> GPMKASLTFSLSGIYAPCSISRDIYLEYGDKKAECLYGTIRLPQYGPGCTPGKIVHCVLDDSLPFCSIVVPSKLFGFMPTQPTMDFCYFEPILDNVVPVLDSVTFLINEQLYSKLMDLPQEMQQIQFLHYKYNINSMETVVHSRDILTSGLCQILN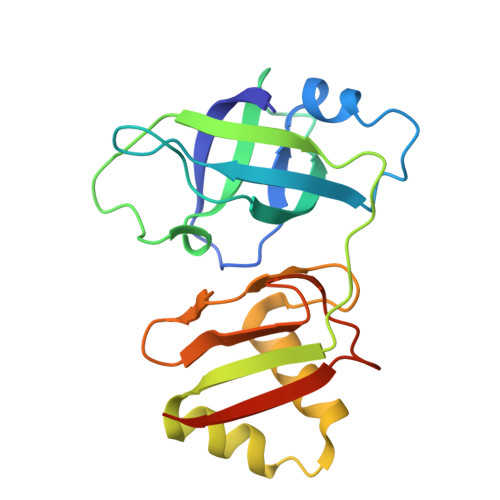CSPFPQGLVDFTETQLILVNDTEQKLSALK> MKVAVLPGDGIGPEVTEAALKVLRALDEAEGLGLAYEVFPFGGAAIDAFGEPFPEPTRKGVEEAEAVLLGSVGGPKWDGLPRKISPETGLLSLRKSQDLFANLRPAKVFPGLERLSPLKEEIARGVDVLIVRELTGGIYFGEPRGMSEAEAWNTERYSKPEV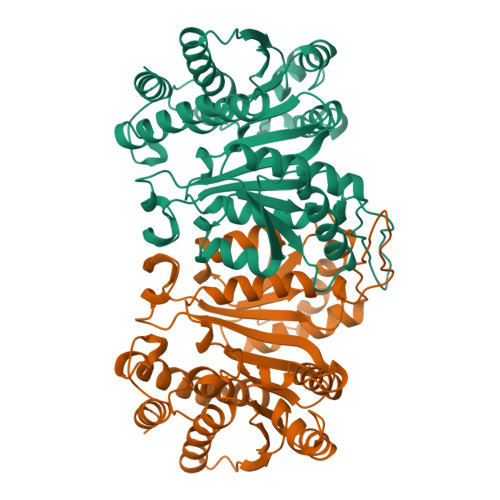ERVARVAFEAARKRRKHVVSVDKANVLEVGEFWRKTVEEVGRGYPDVALEHQYVDAAAMHLVRSPARFDVVVTGNIFGDILSDLASVLPGSLGLLPSASLGRGTPVFEPVHGSAPDIAGKGIANPTAAILSAAMMLEHAFGLVELARKVEDAVAKALLETPPPDLGGSAGTEAFTATVLRHLA>SNATNPTATPLVYKKLSLELPAKTDDLETQLKVYLTANGVQLSNDNDAYVLRVLEYTPRRQLLNGKLTEVLLRLTVT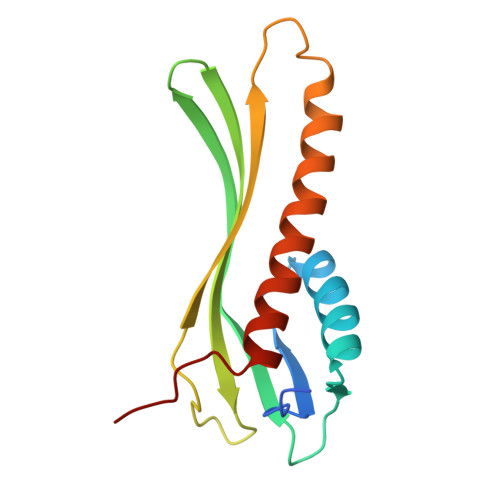FQIEDRQGNKITEPRTLTAARSYQYDLATVNTENQQESYLQRIVIDDLAQQITRQISANRLPKAQP[3x]>MQGVNIYNISAGTSVDLAAPVTTGDIVTFFSSALNLNAGAGNPNNTTLNLFAENGAYLLQIAFRLQENVIIFNSRQPDGPWLVEQRVSDVANQFAGIDGKAMVTVFDHGDKYQVVINEKTVIQYTKQISGLTSSLSYNATEETSIFSTVVEAVTYTGLALEHHH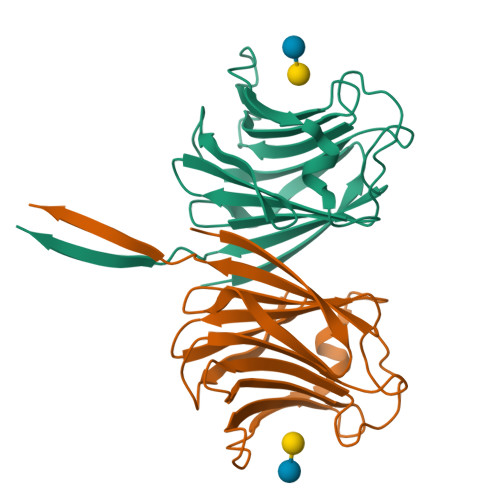HHH[2x]> MQQANLGDGVATARLLSRSDWGARLPKSVEHFQGPAPYVIIHHSYMPAVCYSTPDCMKSMRDMQDFHQLERGWNDIGYSFGIGGDGMIYTGRGFNVIGAHAPKYNDKSVGIVLIGDWRTELPPKQMLDAAKNLIAFGVFKG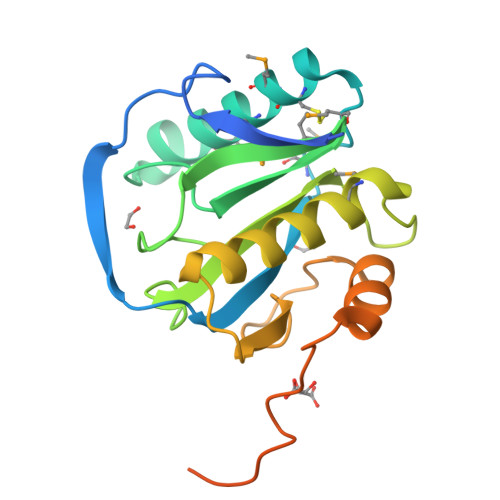YIDPAYKLLGHRQVRDTECPGGRLFAEISSWPHFTHINDTEGVSSTTAPVVPHVHPQAAAPQKPHQSPPAAPKV> MGSSHHHHHHSSGENLYFQGHMEAIQTHPANAAQAKAFTAPGSLSFPGGASEIANSTAPTNGASNGGQQQGVQATSGAGVTPATPAATPGAGPAGPSGITPTLQNIVATVNLDCRLDLKTIALHARNAEYNPKRFAAVIMRIREPKTTALIFASGKMVVTGAKSEDDSKLASRKYARIIQKLGFNAKFTDFKIQNIVGSCDIKFPIRLEGLASKHHNFSSYEPELFPGLIYRMIKPKIVLLIFVSGKIVLTGAKVREEIYQAFEMIYPVLQDFRKV;> MATRLDRLVTILETGSTRLIRDTAVNQLADWQKQHPEELFNLLSRVVPYLRHKDWETRTTAAKAIGKIIENAPLYDPNAGQDEAAPEPTNGSFEVKKEEEKDVLEQDNFFRLESLDVATIVKYGRPLLRGGPVDYNLAALDPQKRLAHLKKTLNGRLGLLGRVFEDEEMPVEQIASPITPNDAAGANGVGRQDGASNDNQSQAIDESKMSARQLNVLKRKRKREAQKAAQGKSGFGDLSLRRSTTAGSDAFGEDTPMPDADSKKNKLAEYFSLDR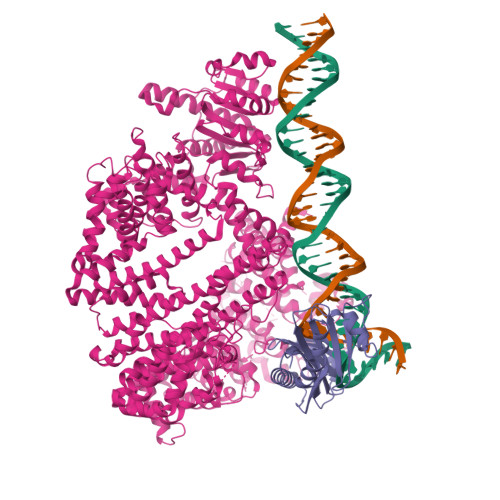PENTEEDTKIVSEFKGPVLPIKSEIEADDSLEGAEWPFERLCEFLKVDLFDPQWETRHGAAMGLREVIRVHGAGAGRRRGKTRKENNDLNRQWLDDLAYRLLCVLMLDKFTDYSSDTSVAPIRETVGQTLGAVLRHISVESVHAIYRLLYCMVTQEDLPSEQNMWAVCHGGMVGLRYVVAVRKDLLLQDGDMIDGVVRCVMQGLGDIDDDVRSVSAATLIPMAKEFVMMRRSALDSLINIVWESLSNLGDDLSASTGKIMDLLATLCSFPEVLEAMKVSASQDEERSFTLLVPRLYPFLRHTITSVRLAVLKALMTFANLGGETSQGWLNGRILRLIFQNIIVERDQDTLNMSLELWTTLVRRLAARDPAILADEFEAHAEPMMQLALHPIGVPRHPIPMNPALFQKPSGGTYSLPGASQTNSRRSSPPEGERATKRRRKSTKAEDVAPSTHTHDVDGHMIQGEVDLVGVDVLIRSRISAAKAMGLIMSFIPTPRLASYDTAVLQALSSPYASTQLAAAMVIDEYAKNCSTPEVASRFIEPLQKIIDLERPSHYRDLVTYVQRVRSASQQLINLFRDHGKVSQGKLPTLAVVVQGEPEAGPGAFSIANAEKVVNEDFERLKRLMAPGQRLIALPQLNEAREQTVEVIEEAKAAKEARDARIKAAAACALVAMKVLPKKPSPLIKAIMDSIKTEENQELQSRSAATIARLVQLFTESGRRGPAEKVVANLVKFSCVEVAETPEFPIHAHKTNVILSMQKEEDRVDHPDAVKYAREAKAARITRRGAKEALEILSKNFGAELLERVPTLRTFMEEPLVRAFSGDLPPEARDPENAFGQEIVDAMSVIRTMTPTLHPALHPFVMQQVPLVIKALRSDLSVFRYMAAKCMATICSVITVDGMTALVEKVLPSINNPLDLSFRQGAIEVIYHLIAVMGDAILPYVIFLIVPVLGRMSDSDNQIRLIATTSFATLVKLVPLEAGIPDPPGLSEELLKGRDRERTFIAQLLDPKKIEPFKIPVAIKAELRSYQQEGVNWLAFLNKYHLHGILCDDMGLGKTLQTICIVASDHHQRAEEFARTGAPEVRKLPSLIICPPTLSGHWQQEIKTYAPFLTVTAYVGSPAERRAMKDSLDKTDIVITSYDVCRNDIDVIEKYNWNYCVLDQGHLIKNPKAKITLAVKRLTSNHRLILTGTPIQNNVLELWSLFDFLMPGFLGAEKVFLDRFAKPIANSRYSKASSKEQEAGALAIEALHKQVLPFLLRRLKEEVLNDLPPKILQNYYCDLSDLQRKLFEDFTKREGKKITETAGRDDKEAKQHIFQALQYMRKLCNSPALVMKPGHKAYEDTQKYLAKHGTTLEDPIHAPKLGALRDLLVDCGIGVEGQESSDPLYTPIKPHRALIFCQMKEMLDMVQNTVLKQMLPSVSYLRLDGSVEANKRQDIVNKFNSDPSYDVLLLTTSVGGLGLNLTGADTVIFVEHDWNPQKDLQAMDRAHRIGQKKVVNVYRIITRGTLEEKILSLQRFKIDVASTVVNQQNAGLATMDTDQILDLFNLGESGPSLITDNKESIEGREEDMVDIETGDVRRPGKKAAWLEGLGELWDNAQYEESFDLDGFLKTMQAAAWSHPQFEK The nuclease NurA and the ATPase/translocase HerA play a vital role in repair of double-strand breaks (DSB) during the homologous recombination in archaea. HerA is a circular ATP-dependent bipolar translocase and helicase; it belongs to the HerA/FtsK bacterial translocases family, an offshoot of the RecA family. Each drHerA protomer comprises three domains: the N-terminal HerA-ATP synthase barrel domain (HAS-barrel domain) that forms the putative exit for the substrate, the RecA-like ATPase domain, and the helix-bundle domain which is inserted into the RecA-like ATPase domain and forms the putative entrance for the substrate. Herein, we characterized, for the first time, the crystal structures of D. radiodurans HerA (drHerA), with and without ADP binding, and a low-resolution cryo-EM structure of the drNurA-HerA complex.

Full-length drHerA without any ligand was crystallized in space group P3121 and the apo structure was solved at 3.0 Å resolution by single-wavelength anomalous diffraction (SAD) phasing using selenomethionine-substituted protein crystals and then refined with the native data. The refined drHerA apo structure contains one hexamer (six protomers) in the asymmetric unit. Not as apo ssoHerA that predominantly exists as a heptamer in solution, drHerA in both nucleotide-free and ADP-binding modes have been crystallized as sixfold symmetrical rings. The shape of the nucleotide-free drHerA hexamer is quite similar to the drHerA-ADP complex, except that the central pore formed by the six subunits is highly symmetric, with a ~28.2 Å inside diameter of the putative DNA translocation motifs, ~24.5 Å inside diameter of the putative DNA entrance, and ~28.5 Å inside diameter of the putative DNA exit. The six N-terminal HAS-barrel domains from the hexamer formed a pore with an approximately 28.5 Å diameter that is large enough for B-form dsDNA threading. A pore with an approximately 24.5 Å diameter was formed by the helix-bundle domains, which is enough for the entry of the B-form dsDNA. Although the last fourteen residues of the C-terminal protrusion are disordered in our drHerA structures, we believe they are too short to stretch into the neighboring protomer. The drHerA apo structure and the predicted drNurA structure were further organized and fitted into the low-resolution cryo-EM map of the drHerA-drNurA complex by Chimera. However, drHerA spontaneously forms a stable hexamer in the absence of DNA or other cofactors. The innate stability of drHerA suggests that drHerA binds the broken DNA spontaneously by threading from the broken end so that the drHerA hexameric ring does not have to be disrupted first.

>[6x]MTGNDVQGAEKADAIGMVLGTEDVTPTVFWFAVSHGASVGLDDLVVVETRKPDGTPVRFYGLVDNVRKRHEGVTFESDVEDVVAGLLPASVSYAARVLVTRVDPENFIPPQPGDHVRHAAGRELAMALSADKMEEAAFPGGLLADGQPLPLNFRFINGESGGHINISGISGVATKTSYALFLLHSIFRSGVMDRTAQGSGGRQSGTAGGRALIFNVKGEDLLFLDKPNARMVEKEDKVVRAKGLSADRYALLGLPAEPFRDVQLLAPPRAGAAGTAIVPQTDQRSEGVTPFVFTIREFCARRMLPYVFSDASASLNLGFVIGNIEEKLFRLAAAQTGKGTGLIVHDWQFEDSETPPENLDFSELGGVNLQTFEQLISYLEYKLLEEREGEGDPKWVLKQSPGTLRAFTRRLRGVQKYLSPLIRGDLTPEQAEGYRPDPLRRGIQLTVVDIHALSAHAQMFVVGVLLREVFEYKERVGRQDTVFVVLDELNKYAPREGDSPIKDVLLDIAERGRSLGIILIGAQQTASEVERRIVSNAAIRVVGRLDLAEAERPEYRFLPQSFRGRAGILQPGTMLVSQPDVPNPVLVNYPFPAWATRRDEVDDLGGKAAAEVGAGLLR To provide a molecular basis for designing better drugs targeting polymerases, African swine fever virus DNA Polymerase X (Pol X) was used as a model for the study. As the simplest DNA polymerase identified to date, Pol X belongs to the polymerase X family and is constituted of 174 amino acids. In this chemical reaction, metal-ion A (MeA) is a catalytic ion and decreases the pKa of 3′-OH, facilitating its attack on the α-phosphate of the incoming dNTP, and metal-ion B (MeB) stabilizes the dNTP-DNA-polymerase complex and increases the electrophilicity of the phosphorus center. To clearly understand the phosphodiester-bond-formation mechanism and the metal-ion catalysis of polymerases, we designed modified dNTP substrates with a chiral α-phosphorus center (α-P center) using a single selenium atom, without affecting the overall and local structures, to explore the absolute configuration inversion and probe the mechanisms of the metal ion–oxygen interactions.

DNApre, generated on the DNA-I by incorporating ddNTP without 3′-OH, failed to attack the incoming dNTP (dGTP, dGTPαSe-I, or dGTPαSe-II), thereby forming the substrate complex (the substrate–primer-template–polymerase complex: nat-dG_sub, dGSe-I_sub, or dGSe-II_sub), resulting in the before-reaction state (without the bond formation) retaining the absolute configuration of dGTPαSe. In crystallization trials, DNApre-I (generated form 5′-CAGGATCCT-3′ with ddTTP, without 3′-OH) and DNApre-II (generated form 5′-CTGGATCCA-3′ with ddATP, without 3′-OH) could not be extended by attacking dGTP or dGTPαSe diastereomers in the crystallization conditions, which allowed the dNTPs to just bind and retain their absolute configuration. Firstly, dGTPαSe diastereomers were synthesized and separated by reversed-phase-HPLC as peak 1 (dGTPαSe-I, eluted first on HPLC) and peak 2 (dGTPαSe-II, eluted later), and their absolute configurations on the α-P center were determined as Rp and Sp, respectively, by X-ray crystallography. Further, when we compared the substrate structures containing native dGTP and dGTPαSe-I, we only found the Se-density difference in the electron map, which indicated the Rp configuration on the Se-modified α-P center, determining the absolute configuration of dGTPαSe-I (Rp diastereomer). As two metal ions occupied the MeA and MeB sites, and they coordinated with the Rp atom in the dGSe-I_sub structure, the electron density on the Rp position was reduced. The distance (in the dGSe-I_sub complex) between the Rp Se atom and MeA (or MeB) was 2.3 Å (or 2.6 Å), while the corresponding one (in native dGTP complex) was 2.0 Å (or 2.1 Å), confirming the interaction between the Se atom and the metal ions. Furthermore, we found that on the phosphonoselenoate group, the P-Se bond length was 1.9 Å (single bond), while the P-O bond length was 1.6 Å (double bond).

>[2x]GGMLTLIQGKKIVNHLRSRLAFEYNGQLIKILSKNIVAVGSLRREEKMLNDVDLLIIVPEKKLLKHVLPNIRIKGLSFSVKVCGERKCVLFIEWEKKTYQLDLFTALAEEKPYAIFHFTGPVSYLIRIRAALKKKNYKLNQYGLFKNQTLVPLKITTEKELIKELGFTYRIPKKRL> MGDEEKKEKKKKSKKKSEEEGGDAAPAPPPPKPPSQKRRAQRSGSNVFAMFTQHQVQEFKEAFQLIDQDKDGFISKNDIRATFDSLGRLCTEQELDSMVAEAPGPINFTMFLTIFGDRIAGTDEEDVIVNAFNLFDEGEGKCKEETLKRSLTTWGEKFSQDEVEEALSEAPIDGNGLIDIKK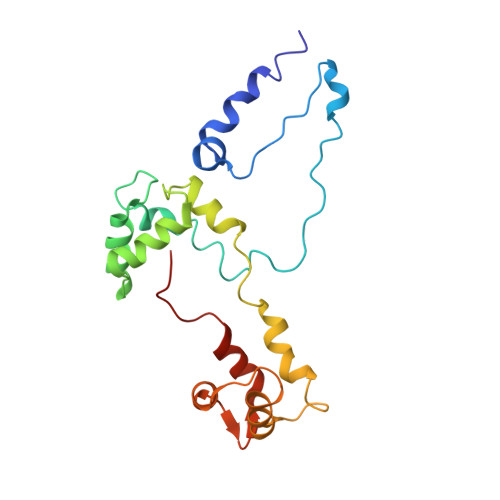FAQILTKGAEEEGA>MSQQVTQLNPTQQTTQSAFLATTVITAQCHAILNTQFTPPTVKPDWFDDLSKKLDSAKLVAKQWIDDLGPQVSASIPSSVINFDATFQASIDAIHELYKADPTASGKDNTTVQQASQIMTALSSQVSGIEATVKGMNKELSDWGVKMQAAHDDLVNGATNIQKTIIDLQTDIESMNNAIDNNRAAIEKLNKDLVYAQVAVGVGIFMLVAGVALTVATAGTAAAVSGGIAAVGAASIIAGGVTWGVLQNQIDDDYDSIAQEQKQKAEDQQQIIALQGLSNASSAVVSAIETSTSVLSDFETTWTVFGNELDDVVTKLNNGASMQSIIMEKVMSDAAKNEWDDAVELAKQLASAKIAIETKELAPAVKQAA[4x]

Using Caenorhabditis elegans and Danio rerio (zebrafish) as host models for bacterial predatory interactions and infection in aqueous environments, respectively, we obtained evidence for a new V. cholerae cytotoxin denoted MakA (motility-associated killing factor A). The crystal structure of MakA revealed that it belongs to the ClyA α-PFT family, named after the potent, one-component, PFT ClyA which is expressed from a monocistronic operon in Escherichia coli. Our recent studies of the proteins encoded by the mak genes in V. cholerae demonstrated that MakA can form a tripartite cytolytic complex with MakB and MakE, whereas neither of the three proteins displays cytolytic activity on their own. Within acidified organelle lumens or when incubated with cells in acidic media, MakA forms oligomers and remodels membranes into high-curvature tubes leading to loss of membrane integrity.

We used helical reconstruction to solve the cryo-EM structure of a MakA filament assembled in vitro in the presence of ECLE liposomes at pH 6.5 and high protein concentrations. One repeating element of the right-handed spiral consists of 37 tetramers that complete five turns around the helical axis, spanning a length of 216.5 Å and a diameter of 322 Å. This arrangement results in an axial rise of 5.85 Å per subunit and a helical twist of 48.65°. Application of these initially calculated values with local searches in a 3D refinement further optimized symmetry parameters and resulted in a cryo-EM map at an overall resolution of 3.7 Å. The building blocks of this filament are formed by two MakA dimers that organize into a pinecone-like architecture, spiraling around a central cavity. From the top view along the filament axis, the helix features a propeller-like structure with a weak, annular density embedded in-between the blades formed by MakA. This density resembles lipid tails and contains some spherical features, which could be associated with phospholipid heads, suggesting the presence of a thin phospholipid bilayer that spirals around the central cavity of the filament. Interestingly, the annular density is located between the TMHs of MakA, indicating that the active toxin form interacts with lipid vesicles and starts to oligomerize by internalizing membrane lipids. Interestingly, despite certain similarities, all four copies of MakA adopt different conformations within the tetramer, as indicated by MakA-1 to MakA-4. In MakA-2 and MakA-4, this region superimposes well with the crystal structure, whereas helix α6 of MakA-1 and MakA-3 moves by almost 10 Å to extend the length of α5.> HHHHHHLESTSLYKKAGFMGVVEEAHNVKVIGSGEATIVLGHGFGTDQSVWKHLVPHLVDDYRVVLYDNMGAGTTNPDYFDFDRYSNLEGYSFDLIAILEDLKIESCIFVGHSVSAMIGVLASLNRPDLFSKIVMISASPRYVNDVDYQGGFEQEDLNQLFEAIRSNYKAWCLGFAPLAVGGDMDSIAVQEFSRTLFNMRPDIALSVGQTIFQSDMRQILPFVTVPCHILQSVKDLAVPVVVSEYLHANLGCESVVEVIPSDGHLPQLSSPDSVIPVILRHIRNDIAM

KARRIKIN INSENSITIVE 2 (KAI2) is an α/β hydrolase involved in seed germination and seedling development. It is essential for plant responses to karrikins, a class of butenolide compounds derived from burnt plant material that are structurally similar to strigolactone plant hormones. The overall fold of KAI2 consists of an α/β hydrolase domain and a four helix cap domain. The active site is present in a largely hydrophobic pocket of volume 336 Å3, with a classical serine hydrolase catalytic triad at its base (composed of Ser95-His246-Asp217).

KAI2 was successfully crystallised from sodium/potassium phosphate in two crystal forms, one orthorhombic, P 21 21 21 (a∼64 Å, b∼66 Å, c∼78 Å) and the other monoclinic, P 21 (a∼50 Å, b∼56 Å, c∼52 Å, β∼116°), each with one protein molecule in the asymmetric unit. Monoclinic KAI2c diffracted to 2.11 Å.> GDQITK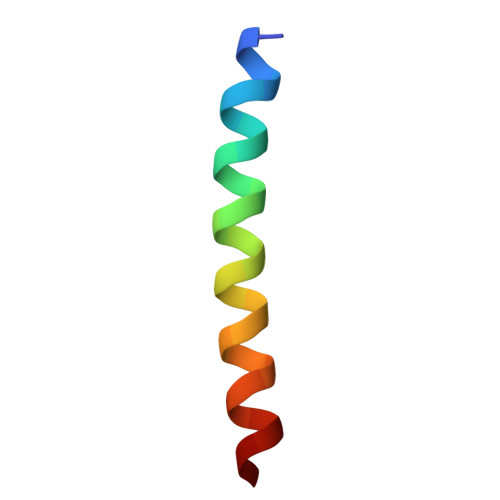MKDRLVEWNDQVEKLGKKMEAR[(2S,3S,4S,5R,6S)-6-[(2R)-2,3-bis(oxidanyl)propoxy]-3,4,5-tris(oxidanyl)oxan-2-yl]methanesulfonic acid | C9 H18 O10 S | 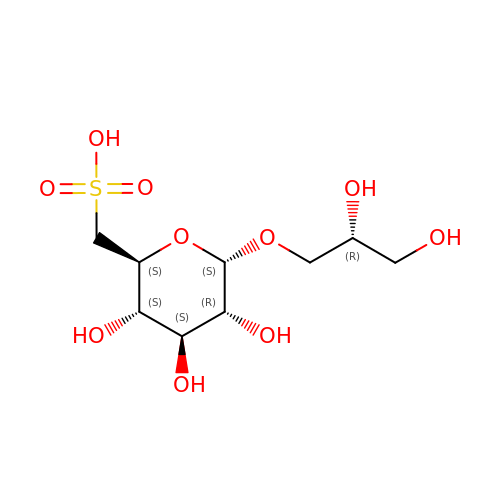JTXHNMDHGMNPEG-NZJLWHDDSA-N>[4x]APKNELVQKFQVYYLGNVPVAKPVGVDVINGALESVLSSSSREQWTPSHVSVAPATLTILHQQTEAVLGECRVRFLSFLAVGRDVHTFAFIMAAGPASFCCHMFWCEPNAASLSEAVQAACMLRYQKCLDARSQHHHHHH

Fe65 is a multidomain protein including an N-terminal α-helical domain and three protein-protein interaction modules: a WW domain and two consecutive C-terminal phosphotyrosine-binding (PTB) domains. Fe65 determines localization and nuclear signaling of APP and modulates APP processing and Aβ-peptide generation. Most attention has been given to Fe65-PTB2 as it directly interacts with the AICD and thus functionally joins the two proteins. Here we present structural and functional data on Fe65-PTB2 revealing the domain as flexible module forming a homodimer in vitro and ex vivo in the absence of APP.

Unspecific aggregation of Fe65-PTB2 at concentrations in the mg/mL range can be prevented by the addition of glycerol and we subsequently crystallized the domain and solved its crystal structure by molecular replacement at 2.6 Å resolution. Fe65-PTB2 crystallizes as dimer of dimers with a continuous central β-sheet. Dimerization occurs via a structural transition of the C-terminal α-helix α3 within one Fe65-PTB2 subunit (the “complementing” subunit) in respect to the conformation as seen in the previously solved AICD/Fe65-PTB2 complex (rmsd of 0.85 Å for 123 Cα-atoms; Radzimanowski et al., 2008c). The last two helical turns dissolve (starting at L656) and adopt an extended β-conformation that complements the “accommodating” subunit in trans (dimer interface: 585 Å2). The newly formed β-strand (defined here as βct) quasi-symmetrically mediates also the dimer of dimer contact with the tetrameric assembly being stabilized by a disulfide bridge between respective cysteine (C661) residues. In the crystal structure of the Fe65-PTB2 dimer, the induced strand βct with the C661LD sequence directly matches to the AICD strand. Thus, the complementing Fe65-PTB2 mimics the interacting AICD in space and charge. In summary, Fe65-PTB2 dimerization results in a structural change that blocks the AICD binding site either fundamentally in the accommodating subunit or partially in the complementing subunit. The analysis revealed a pronounced positively charged patch (R605, R607, R657, K660 and R665) in the center of the dimer directly located at the transition site of the C-terminal helix. Most strikingly, in the elongated patch next to the dimer interface we find three adjacent sulfate ions.> AQSVPYGVSQIKAPALHSQGYTGSNVKVAVIDSGIDSSHPDLKVAGGASMVPSETNPFQDNNSHGTHVAGTVAALNNSIGVLGVAPSASLYAVKVLGADGSGQYSWIINGIEWAIANNMDVINMSLGGPSGSAALKAAVDKAVASGVVVVAAAGNEGTSGSSSTVGYPGKYPSVIAVGAVDSSNQRASFSSVGPELDVMAPGVSIQSTLPGNKYGAYNGTSMASPHVAGAAALILSKHPNWTNTQVRSSLQ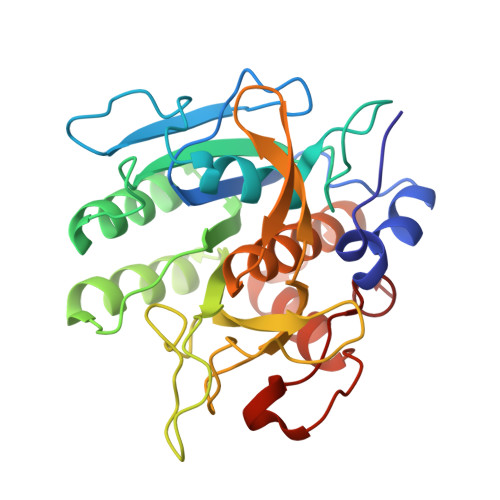NTTTKLGDSFYYGKGLINVQAAAQ> MELIQDTSRPPLEYVKGVPLIKYFAEALGPLQSFQARPDDLLISTYPKSGTTWVSQ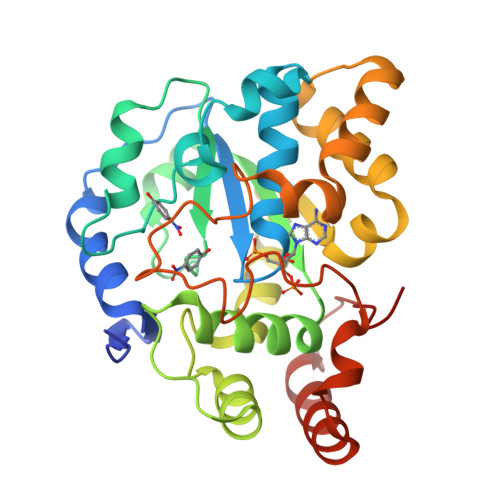ILDMIYQGGDLEKCHRAPIFMRVPFLEFKAPGIPSGMETLKDTPAPRLLKTHLPLALLPQTLLDQKVKVVYVARNAKDVAVSYYHFYHMAKVHPEPGTWDSFLEKFMVGEVSYGSWYQHVQEWWELSRTHPVLYLFYEDMKENPKREIQKILEFVGHSLPEETVDFMVQHTSFKEMKKNPMTNYTTVPQEFMDHSISPFMRKGMAGDWKTTFTVAQNERFDADYAEKMAGCSLSFRSEL> MATKAARVPRTVLPFEAMPRRPGNRRNRLNQIRREQGYEDLHLEVHQTFQELGPIFRYDLGGAGMVCVMLPEDVEKLQQVDSLHPHRMSLEPWVAYRQHRGHKCGVFLLNGPEWRFNRLRLNPEVLSPNAVQRFLPMVDAVARDFSQALKKKVLQNARGSLTLDVQPSIFHYTIEASNLALFGERLGLVGHSPSSASLNFLHALEVMFKSTVQLMFMPRSNSRNTSPKVWKEHFEAWDCIFQYGDNCIQKIYQELAFSRPQQYTS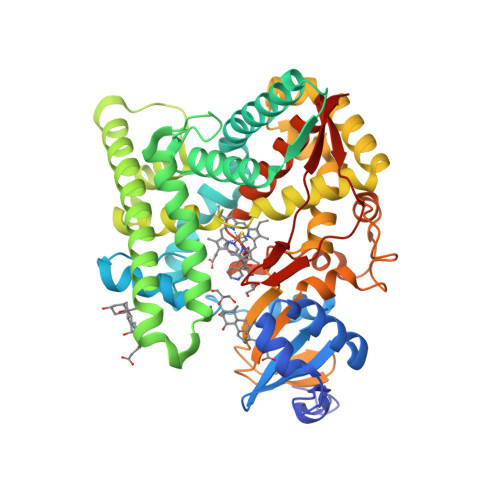IVAELLLNAELSPDAIKANSMELTAGSVDTTVFPLLMTLFELARNPNVQQALRQESLAAAASISEHPQKATTELPLLRAALKETLRLYPVGLFLERVASSDLVLQNYHIPAGTLVRVFLYSLGRNPALFPRPERYNPQRWLDIRGSGRNFYHVPFGFGMRQCLGRRLAEAEMLLLLHHVLKHLQVETLTQEDIKMVYSFILRPSMFPLLTFRAINHHHHHH4-[4-[(4,4-dimethylpiperidin-1-yl)methyl]phenyl]-9-[6-[(phenylmethyl)amino]pyrimidin-4-yl]-1,4,9-triazaspiro[5.5]undecan-2-one 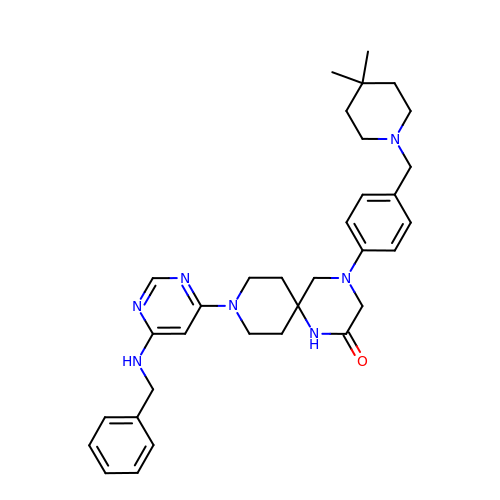| C33 H43 N7 O | SMOMNPRYHLVUTG-UHFFFAOYSA-N The yeast lipid flippase Drs2p-Cdc50p is primarily found in the trans-Golgi network and is involved in protein trafficking between that network, the plasma membrane, and endosomes. Drs2p belongs to a large family of Type IV P-type ATPases (P4 ATPases). These enzymes translocate specific phospholipids from the extracellular side of the plasma membrane or from the lumenal side of internal organelles to the cytosolic side, creating and maintaining lipid compositional asymmetry in eukaryotic cell membranes. Drs2p-Cdc50p is activated by the binding of phosphatidylinositol 4-phosphate (PI4P), the Arf guanine nucleotide exchange factor Gea2p, and the Arf-related small-GTP-binding protein Arl1p to the C-terminal region of Drs2p9,10.

After 2D and 3D classifications, some 640,000 particles were selected for 3D reconstruction and refinement, leading to a 3D map in the apo form at 2.8 Å resolution. We found the purified Drs2p-Cdc50p was free of any ligand in an autoinhibited apo state. In our apo Drs2p structure, the ordered region of the Drs2p C-tail is 57 residues long and fills an extended horizontal groove between the second-tier A and P domains and the third-tier N domain. Hence, the Drs2p C-tail makes extensive contact with all three cytosolic regulatory domains. A structural alignment with the SERCA ATPase in complex with ATP showed that the nucleotide-binding site was occluded by Phe-1275 and Phe-1277 in the C-tail. The C-tail appears to cement the A, N, and P domains, preventing ATP binding by inserting these two phenylalanine residues into the nucleotide pocket and physically separating the N domain from the P domain, so that Asp-560 of the P domain cannot be phosphorylated. This structural feature readily explains why Drs2p in the apo form is fully inhibited by its C-tail. The ordered N-terminal peptide extends over both the P and A domains. In particular, this N-peptide engages in two hydrophobic interactions with the A domain, one involving Ile-203 of the N-peptide and Leu-427 and His-422 of A domain, and the other involving Tyr-198 of the N-peptide and Val-304 of A domain. These interactions likely account for the observed inhibitory effect of the N-terminus on Drs2p activity. We suggest the apo Drs2p is in a unique autoinhibited conformation that is distinct from any of the four active states of the SERCA ATPase.

> MNDDRETPPKRKPGEDDTLFDIDFLDDTTSHSGSRSKVTNSHANANYIPPSHVLPEETIDLDADDDNIENDVHENLFMSNNHDDQTSWNANRFDSDAYQPQSLRAVKPPGLFARFGNGLKNAFTFKRKKGPESFEMNHYNAVTNNELDDNYLDSRNKFNIKILFNRYILRKNVGDAEGNGEPRVIHINDSLANSSFGYSDNHISTTKYNFATFLPKFLFQEFSKYANLFFLCTSAIQQVPHVSPTNRYTTIGTLLVVLIVSAMKECIEDIKRANSDKELNNSTAEIFSEAHDDFVEKRWIDIRVGDIIRVKSEEPIPADTIILSSSEPEGLCYIETANLDGETNLKIKQSRVETAKFIDVKTLKNMNGKVVSEQPNSSLYTYEGTMTLNDRQIPLSPDQMILRGATLRNTAWIFGLVIFTGHETKLLRNATATPIKRTAVEKIINRQIIALFTVLIVLILISSIGNVIMSTADAKHLSYLYLEGTNKAGLFFKDFLTFWILFSNLVPISLFVTVELIKYYQAFMIGSDLDLYYEKTDTPTVVRTSSLVEELGQIEYIFSDKTGTLTRNIMEFKSCSIAGHCYDDKIPEDKTATVEDGIEVGYRKFDDLKKKLNDPSDEDSPIINDFLTLLATCHTVIPEFQSDGSIKYQAASPDEGALVQGGADLGYKFIIRKPNSVTVLLEETGEEKEYQLLNICEFNSTRKRMSAIFRFPDGSIKLFCKGADTVILERLDDEANQYVEATMRHLEDYASEGLRTLCLAMRDISEGEYEEWNSIYNEAATTLDNRAEKLDEAANLIEKNLILIGATAIEDKLQDGVPETIHTLQEAGIKIWVLTGDRQETAINIGMSCRLLSEDMNLLIINEETRDDTERNLLEKINALNEHQLSTHDMNTLALVIDGKSLGFALEPELEDYLLTVAKLCKAVICCRVSPLQKALVVKMVKRKSSSLLLAIGDGANDVSMIQAAHVGVGISGMEGMQAARSADIAVGQFKFLKKLLLVHGSWSYQRISVAILYSFYKNTALYMTQFWYVFANAFSGQSIMESWTMSFYNLFFTVWPPFVIGVFDQFVSSRLLERYPQLYKLGQKGQFFSVYIFWGWIINGFFHSAIVFIGTILIYRYGFALNMHGELADHWSWGVTVYTTSVIIVLGKAALVTNQWTKFTLIAIPGSLLFWLIFFPIYASIFPHANISREYYGVVKHTYGSGVFWLTLIVLPIFALVRDFLWKYYKRMYEPETYHVIQEMQKYNISDSRPHVQQFQNAIRKVRQVQRMKKQRGFAFSQAEEGGQEKIVRMYDTTQKRGKYGELQDASANPFNDNNGLGSNDFESAEPFIENPFADGNQNSNRFSSSRDDISFDI;> MVSLFKRGKAPPLTKEGPTSKKPPNTAFRQQRLKAWQPILSPQSVLPLLIFVACIFTPIGIGLIVSATKVQDLTIDYSHCDTKASTTAFEDIPKKYIKYHFKSKVENKPQWRLTENENGEQSCELQFEIPNDIKKSIFIYYKITNFYQNHRRYVQSFDTKQILGEPIKKDDLDTSCSPIRSREDKIIYPCGLIANSMFNDTFSQVLSGIDDTEDYNLTNKHISWSIDRHRFKTTKYNASDIVPPPNWMKKYPDGYTDENLPDIHTWEEFQVWMRTAAFPKFYKLTLKNESASLPKGKYQMNIELNYPISLFGGTKSFVLTTNGAIGGRNMSLGVLYLIVAGLCALFGIIFLVKLIFQPRAMGDHTYLNFDDEENEDYEDVHAENTTLREIL> TCPSRCTCSGDSLDCGGRGLAALPGDLPSSTRSLNLSYNKLSEIDPAGFEDLPNLQEVYLNNNELTAVPSLGAASSHVVSLFLQHNKIRSVEGSQLKAYLSLEVLDLSLNNITEVRNTCFPHGPPIKELNLAGNRIGTLELGAFDGLSRSLLTLRLSKNRITQLPVRAFKLPRLTQLDLNRNRIRLIEGLTFQGLNSLEVLKLQRNNISKLTDGAFWGLSKMHVLHLEYNSLVEVNSGSLYGLTALHQLHLSNNSIARIHRKGWSFCQKLHELVLSFNNLTRLDEESLAEL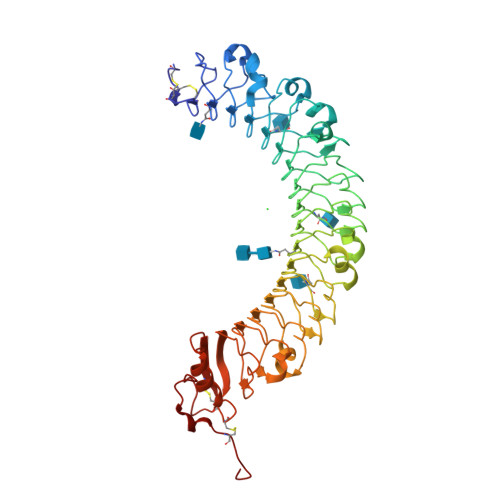SSLSVLRLSHNSISHIAEGAFKGLRSLRVLDLDHNEISGTIEDTSGAFSGLDSLSKLTLFGNKIKSVAKRAFSGLEGLEHLNLGGNAIRSVQFDAFVKMKNLKELHISSDSFLCDCQLKWLPPWLIGRMLQAFVTATCAHPESLKGQSIFSVPPESFVCDDFLKA>[4x]MAVPETRPNHTIYINNLNEKIKKD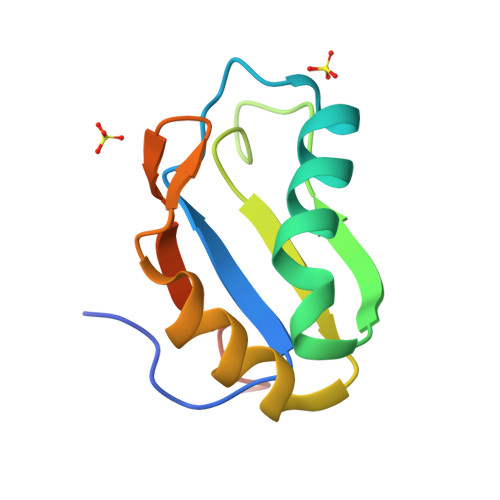ELKKSLHAIFSRFGQILDILVSRSLKMRGQAFVIFKEVSSATNALWSMQGFPFYDKPMRIQYAKTDSDIIAKMW>VDGDQCESN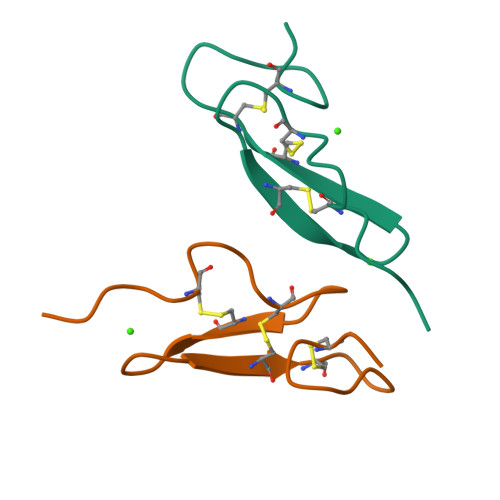PCLNGGSCKDDINSYECWCPFGFEGKNCEL[2x]>TSAVLLDHCHFSQVIFNSVEKFYIPGGDVTCHY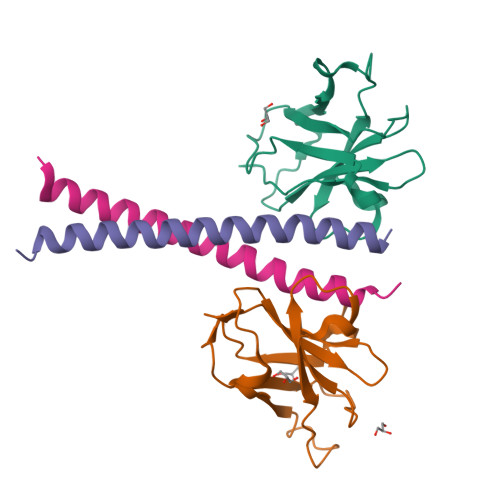TFTQHFIPRRKDWIGIFRVGWKTTREYYTFMWVTLPIDLNNKSAKQQEVQFKAYYLPKDDEYYQFCYVDEDGVVRGASIPFQFR[2x];>[2x]ESVASHFALVTAYEDIKKRLKDSEKENSLLKKRIRFLEEKLIA> MNNLYRELAPVTDEAWGEIEQEATRTFKRHIAGRRVVDCTGPTGATTAAVSTGHLLDVTSPGDGVIAHLRDSRPLVRLRVPFTITRDAIDDVERGSQDSDWDPVKDAAKKLAFAEDRAIFEGYAAANIQGIRAGSSNPGLALPDDPRGYPDVIAQALSELRLAGVDGPYSVLLSADAYTKVSETTEHGYPLREHLNRVVDGDIIWAPAIDGAFVLS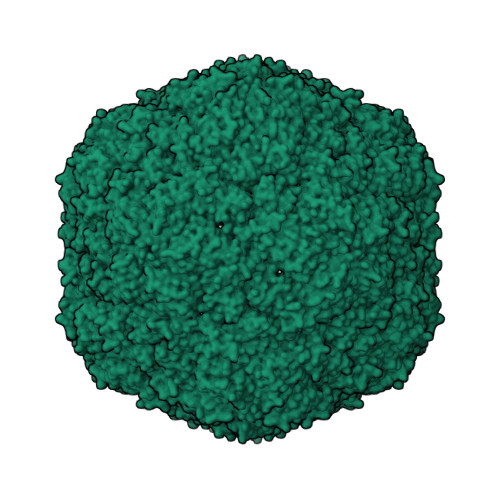TRGGDFDLQLGTDVSIGYSSHDADTVQLYLQETFTFLNYTAEASVALSA> QCDVPPNSRFDCAPDKAITQEQCEARGCCYIPAKQGLQGAQMGQPWCFFPPSYPSYKLENLSSSEMGYTATLTRTTPTFFPKDILTLRLDVMMETENRLHFTIKDPANRRYEVPLETPRVHSRAPSPLYSVEFSEEPFGVIVHRQLDGRVLLNTTVAPLFFADQFLQLSTSLPSQYITGLAEHLSPLMLSTSWTRITLWNRDLAPTPGANLYGSHPFYLALEDGGSAHGVFLLNSNAMDVVLQPSPA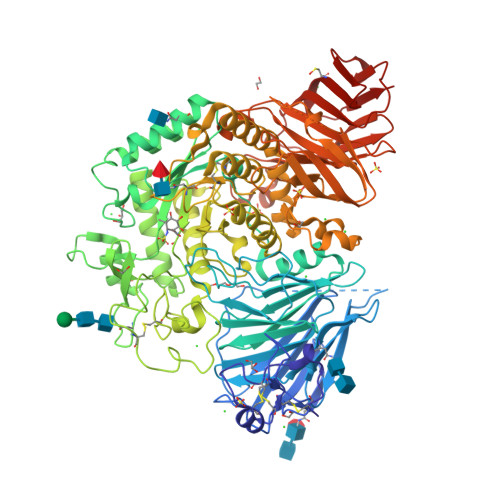LSWRSTGGILDVYIFLGPEPKSVVQQYLDVVGYPFMPPYWGLGFHLCRWGYSSTAITRQVVENMTRAHFPLDVQWNDLDYMDSRRDFTFNKDGFRDFPAMVQELHQGGRRYMMIVDPAISSSGPAGSYRPYDEGLRRGVFITNETGQPLIGKVWPGSTAFPDFTNPTALAWWEDMVAEFHDQVPFDGMWIDMNEPSNFIRGSEDGCPNNELENPPYVPGVVGGTLQAATICASSHQFLSTHYNLHNLYGLTEAIASHRALVKARGTRPFVISRSTFAGHGRYAGHWTGDVWSSWEQLASSVPEILQFNLLGVPLVGADVCGFLGNTSEELCVRWTQLGAFYPFMRNHNSLLSLPQEPYSFSEPAQQAMRKALTLRYALLPHLYTLFHQAHVAGETVARPLFLEFPKDSSTWTVDHQLLWGEALLITPVLQAGKAEVTGYFPLGTWYDLQTVPIEALGSLPPPPAAPREPAIHSEGQWVTLPAPLDTINVHLRAGYIIPLQGPGLTTTESRQQPMALAVALTKGGEARGELFWDDGESLEVLERGAYTQVIFLARNNTIVNELVRVTSEGAGLQLQKVTVLGVATAPQQVLSNGVPVSNFTYSPDTKVLDICVSLLMGEQFLVSWC> MAHHHHHHMKNFFESPFKGKIIK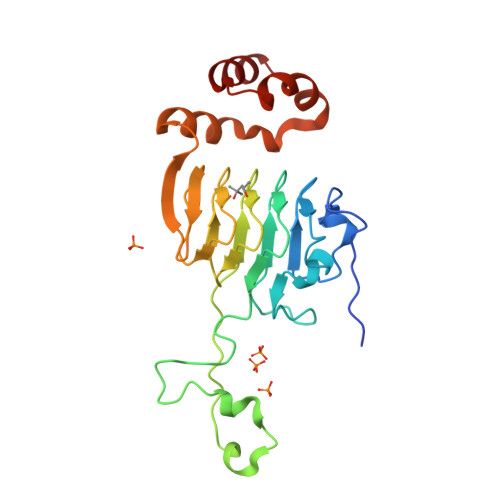DHIQNPNIIAGKYSYYSGYYHGHSFDDCARYLLPDRNDVDKLIIGSYCSVGTGASFIMAGNQGHRYDWISSFPFFYMNEVEAFENSIDAFKNAGDTIIGNDVWIGGEAMIMPGIKIGDGAVIGSRALVTKDVEPYAIVGGNPAKLIKKRFSENQIAILLEIKWWEWNEEVLADAMPILCSGNIDLLYKFYKNI>MRHPLVMGNWKLNGSRHMVHELVSNLRKELAGVAGCAVAIAPPEMYIDMAKREAEGSHIMLGAQNVNLNLSGAFTGETSAAMLKDIGAQYIIIGHSERRTYHKESDELIAKKFAVLKEQGLTPVLCIGETEAENEAGKTEEVCARQIDAVLKTQGAAAFEGAVIAYEPVWAIGTGKSATPAQAQAVHKFIRDHIAKVDANIAEQVIIQYGGSVNASNAAELF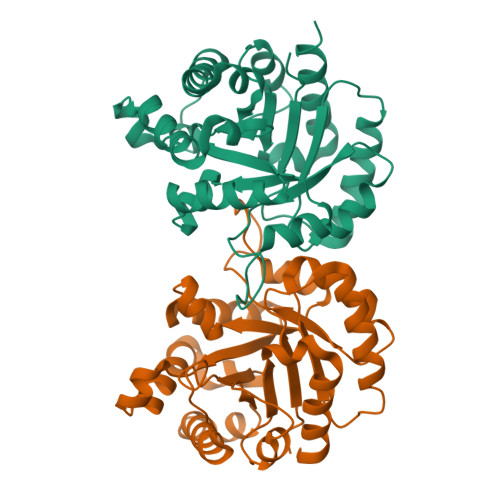AQPDIDGALVGGASLKADAFAVIVKAAEAAKQA[2x]> GSHMSGIALSRLAQERKAWRKDHPFGFVAVPTKNPDGTMNLMNWECAIPGKKGTPWEGGLFKLRMLFKDDYPSSPPKCKFEPPLFHPNVAPSGTVCLSILEEDKDWR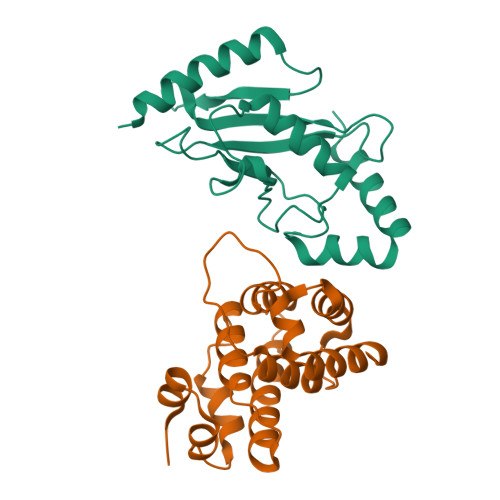PAITIKQILLGIQELLNEPNIQDPAQAEAYTIYCQNRVEYEKRVRAQAKKFAPS;> STGEPAPVLSSPPPADVSTFLAFPSPEKLLRLGPKSSVLIAQQTDTSDPEKVVSAFLKVSSVFKDEATVRMAVQDAVDALMQKAFNSSSFNSNTFLTRLLVHMGLLKSEDKVKAIANLYGPLMALNHMVQQDYFPKALAPLLLAFVTKPNSALESCSFARHSLLQTLYKV>[2x]MAEQLLPQALYLSNMRKAVKIRERTPEDIFKPTNGIIYHFKTMHRYTLEMFRTCQFCPQFREIIHKALIDRSVQASLESQKKLNWCREVRKLVALKTNGDGNCLMHAACQYMWGVQDTDLVLRKALCSTLKETDTRNFKFRWQLESLKSQEFVETGLCYDTRNWNDEWDNLVKMASADTPAARSGLQYNSLEEIHIFVLSNILRRPIIVISDKMLRSLESGSNFAPLKVGGIYLPLHWPAQECYRYP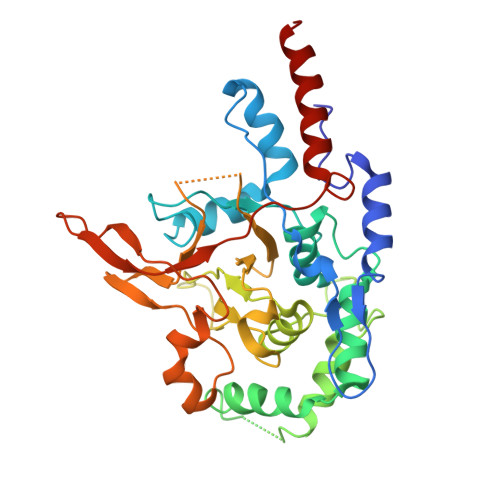IVLGYDSQHFVPLVTLKDSGPELRAVPLVNRDRGRFEDLKVHFLTDPENEMKEKLLKEYLIVMEIPVQGWDHGTTHLINAAKLDEANLPKEINLVDDYFELVQHEYKKWQENS>MHLYSSDFPLMMDEKELYEKWMRTVEMLKAEGIIRSKEVERAFLKYPRYLSVEDKYKKYAHIDEPLPIPAGQTVSAPHMVAIMLEIANLKPGMNILEVGTGSGWNAALISEIVKTDVYTIERIPELVEFAKRNLERAGVKNVHVILGDGSKGFPPKAPYDVIIVTAGAPKIPEPLIEQLKIGGKLIIPVGSYHLW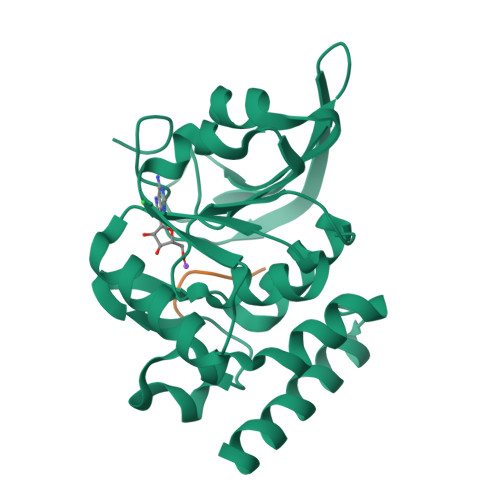QELLEVRKTKDGIKIKNHGGVAFVPLIGEYGWKEHHHHHH[2x];>[2x]VYPDHA> KFDDVCGCDEARAELEEIVDFLKDPTKYESLGGKLPKGVLLTGPPGTGKTLLARATAGEAGVDFFFMSGSEFDEVYVGVGAKRIRDLFAQARSRAPAIIFIDQLDAIGGKRNPKDQAYAKQTLNQLLVELDGFSQTSGIIIIGATNFPEALDKALTRPGRFDKVVNVDLPDVRGRADILKHHMKKITLADNVDPTIIARGTPGLSGAELANLVNQAAVYACQKNAVSVDMSHFEWAKDKILMGAERKTMVLTDAARKATAFHEAGHAIMAKYTNGATPLYKATILPRGRALGITFQLPEMDKVDITKRECQARLDVCMGGKIAEELIYGKDNTTSGCGSDLQSATGTARAMVTQYGMSDDVGPVNLSEEWESWSNKIRDIADNEVIELLKDSEERARRLLTKKNVELHRLAQGLIEYETLDAHEIE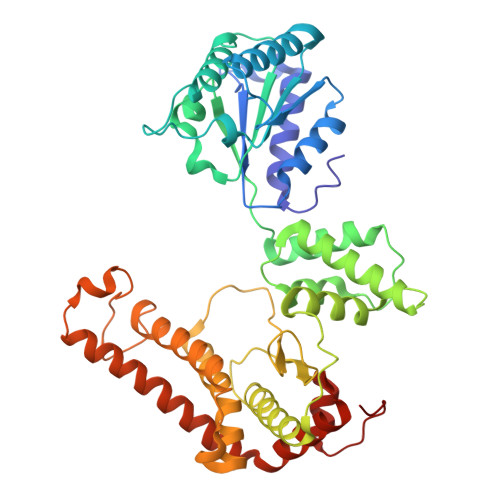QVCKGEKLAKLKT>MDFYYLPGSAPCRAVQMTAAAVGVELNLKLTNLMAGEHMKPEFLKLNPQHCIPTLVDEDGFVLWESRAIQIYLVEKYGAHDADLAERLYPSDPRRRAVVHQRLFFDVAVLYQRFAEYYYPQIFGQKVPVGDPGRLRSMEQALEFLNTFLE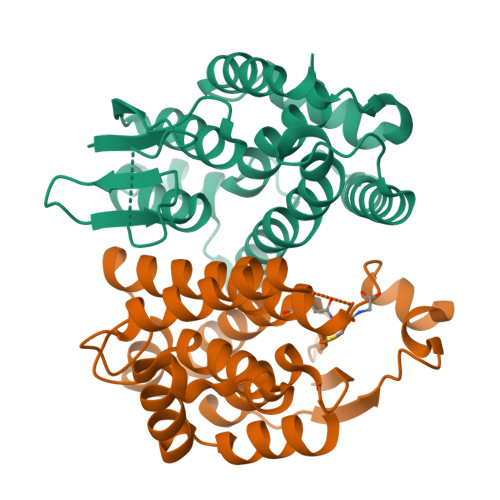GEQYVAGGDDPTIADLSILATIATYEVAGYDLRRYENVQRWYERTSAIVPGADKNVEGAKVFGRYFTQK[2x]cycloheptanamine | C7 H15 N | 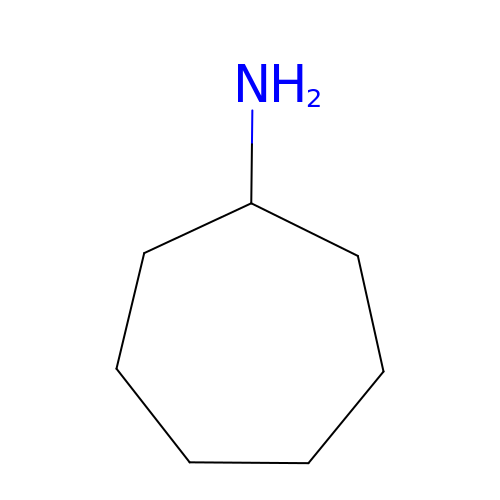VXVVUHQULXCUPF-UHFFFAOYSA-N> SMMELRVGNRYRLGRKIGSGSFGDIYLGTDIAAGEEVAIKLECVKTKHPQLHIESKIYKMMQGGVGIPTIRWCGAEGDYNVMVMELLGPSLEDLFNFCSRKFSLKTVLLLADQMISRIEYIHSKNFIHRDVKPDNFLMGLGKKGNLVYIIDFGLAKKYRDARTHQHIPYRENKNLT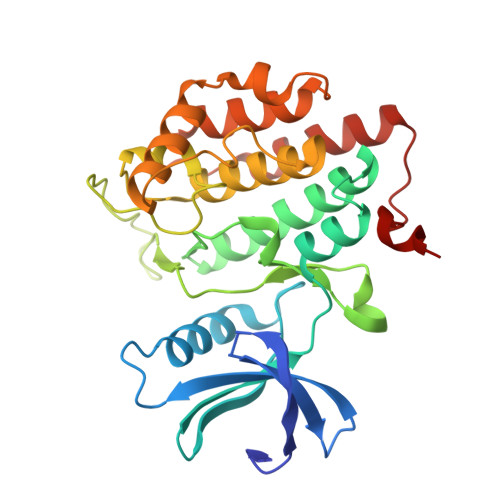GTARYASINTHLGIEQSRRDDLESLGYVLMYFNLGSLPWQGLKAATKRQKYERISEKKMSTPIEVLCKGYPSEFATYLNFCRSLRFDDKPDYSYLRQLFRNLFHRQGFSYDYVFDWNMLK> MELIRIAMKKDLENDNSLMNKWATVAGLKNPNPLYDFLNHDGKTFNEFSSIVNIVKSQYPDREYELMKDYCLNLDVKTKAARSALEYADANMFFEIEDVLIDSMISCSNMKSKEYGKVYKIHRELSNSVITEFEAVKRLGKLNIKTPEMNSFSRLLLLYHYLSTGNFSPMAQLIKQIDLSEISENMYIRNTYQTRVHVLMSNIKLNENSLEECREYSKKALESTNILRFQVFSYLTIGNSLLFSNYELAQENFLKGLSISVQNENYNMIFQQALCFLNNVWRKENKWINFESDSIMDLQEQAHCFINFNE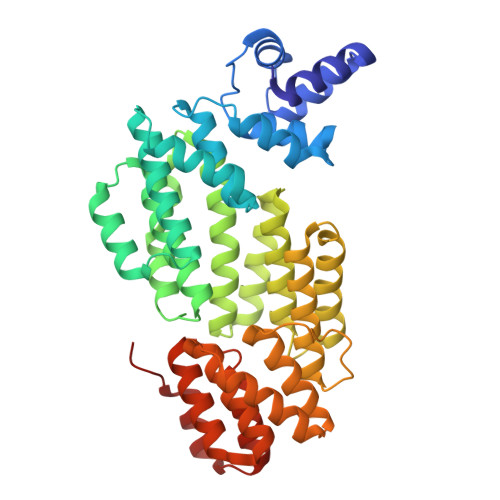NSKAKEVLDKLDLLVHNDNELAMHYYLKGRLEQNKACFYSSIEYFKKSNDKFLIRLPLLELQKMGENQKLLELLLLLEHHH>SVVLPVAKRGEDILKLIAAPVSANELNSNWLYQLADAMHATMLERNGVGIAAPQVYISKRVIIVASRPNPRYPDAPEMNAVVMVNPEILEFSSETCLGEEGCLSVPDERGQVERAEMVKVKYLTLQGEAVETIFHGFPARIVQHEVDHLNGILFVER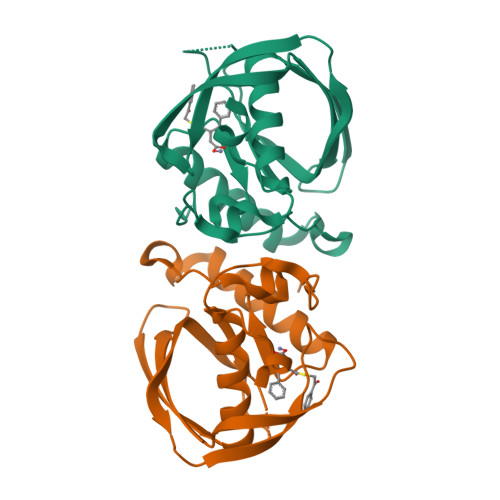IS[2x]5-[2-(4,4-dimethyl-2-oxidanylidene-pyrrolidin-1-yl)ethoxy]-2-fluoranyl-benzenecarbonitrile 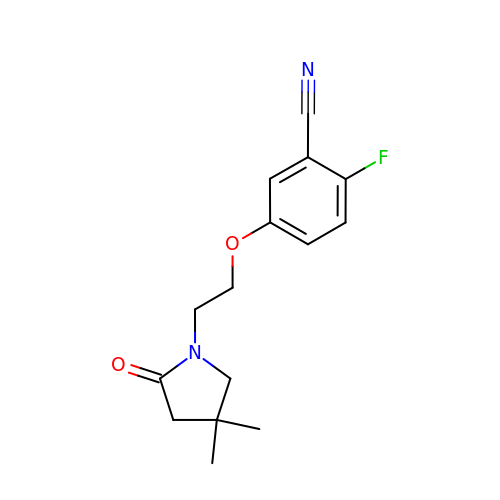| C15 H17 F N2 O2 | GRUADGBFIDAGDY-UHFFFAOYSA-N> SGSWQTYVDEHLMCDIEGTGQHLASAAIFGTDGNVWAKSSSFPEFKPDEINAIIKEFSEPGALAPTGLFLAGAKYMVIQGEPGAVIRGKKGAGGI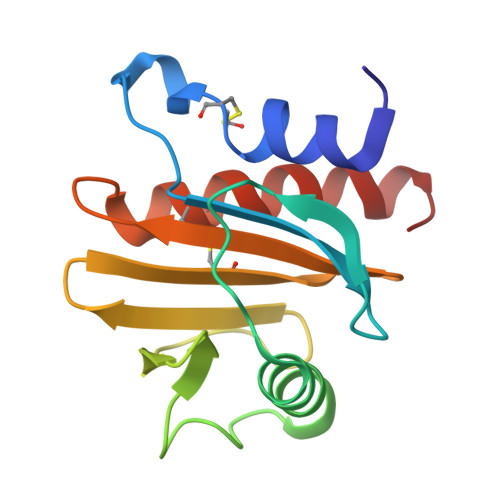CIKKTGQAMVFGIYEEPVNPGQCNMVVERLGDYLVDQGM>MLVGLIGYGAIGKFLAEWLERNGFEIAAILDVRGEHEKMVRGIDEFLQREMDVAVEAASQQAVKDYAEKILKAGIDLIVLSTGAFADRDFLSRVREVCRKTGRRVYIASGAIGGLDAIFSASELIEEIVLTTRKNWRQFGRKGVIFEGSASEA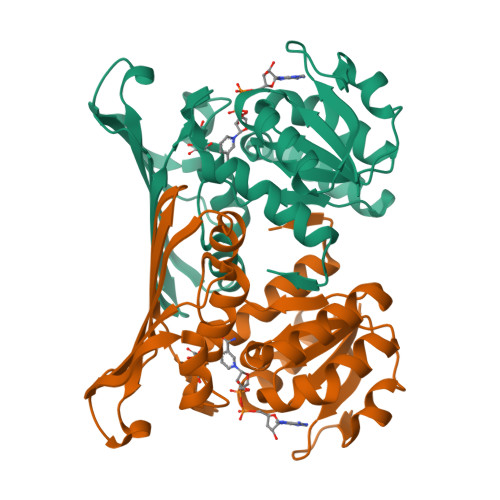AQKFPKNLNVAATLSIASGKDVKVRLVADEVEENIHEILVRGEFGEMEIRVRNRPMRENPKTSYLAALSVTRILRNLKEGLVV[2x]> MAQVLRGTVTDFPGFDERADAETLRKAMKGLGTDEESILTLLTSRSNAQRQEISAAFKTLFGRDLLDDLKSELTGKFEKLIVALMKPSRLYDAYELKHALKGAGTNEKVLTEIIASRTPEELRAIKQVYEEEYGSSLEDDVVGDTSGYYQRMLVVLLQANRDPDAGIDEAQVEQDAQALFQAGELKWGTDEEKFITIFGTRSVSHLRKVFDKYMTISGFQIEETIDRETSGNLEQLLLAVVKSIRSIPAYLAETLYYAMKGAGTDDHTLIRVMVSRSEIDLFNIRKEFRKNFATSLY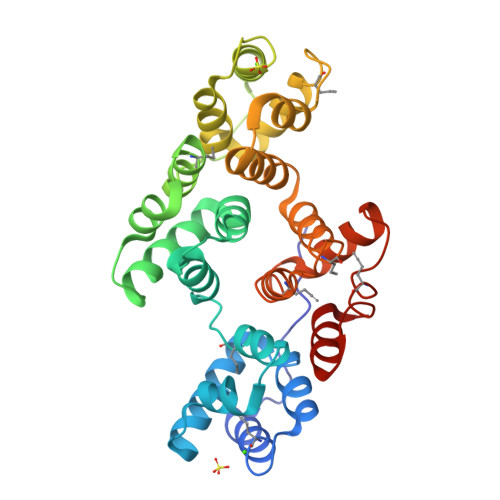SMIKGDTSGDYKKALLLLCGEDD> GGLEKDFL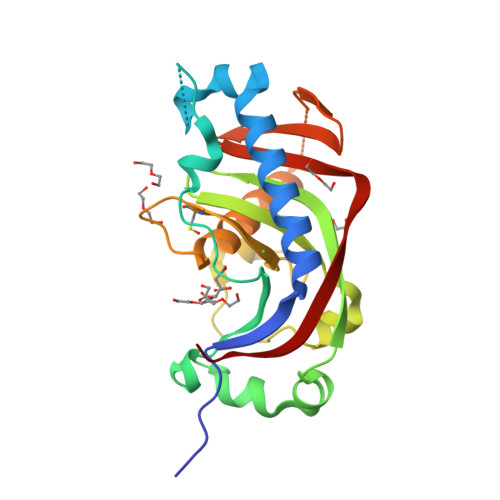PLYFGWFLTKKSSETLRKAGQVFLEELGNHKAFKKELRHFISGDEPKEKLELVSYFGKRPPGVLQCTTKFCDYGKAAGAEEYAQQEVVKRSYGKAFKLSISALFVTPKTAGAQVVLTDQELQLWPSDLDKPSASEGLPPGSRAHVTLGCAADVQPVQTGLDLLDILQQVKGGSQGEAVGELPRGKLYSLGKGRWMLSLTKKMEVKAIFTGYYG(3~{R},3'~{S})-4-methyl-3'-phenyl-spiro[1~{H}-1,4-benzodiazepine-3,2'-oxirane]-2,5-dione 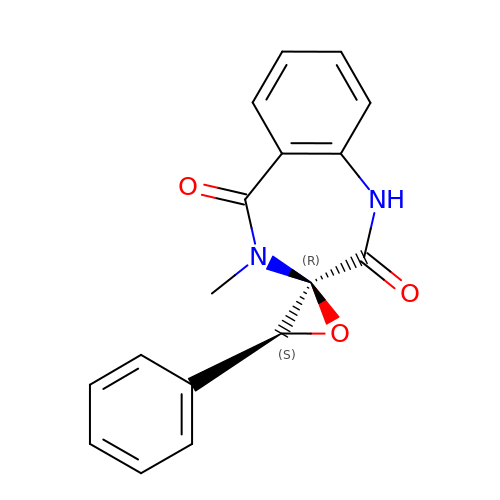| C17 H14 N2 O3 | APLKWZASYUZSBL-WMLDXEAASA-N>[2x]MAVERTLIIVKPDAMEKGALGKILDRFIQEGFQIKALKMFRFTPEKAGEFYYVHRERPFFQELVEFMSSGPVVAAVLEGEDAIKRVREIIGPTDSEEARKV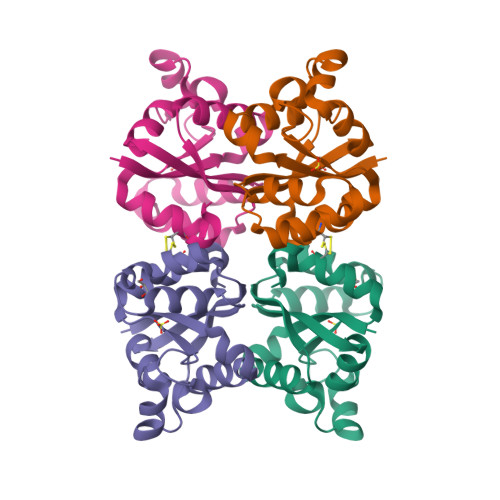APNSIRAQFGTDKGKNAIHASDSPESAQYEICFIFSGLEIV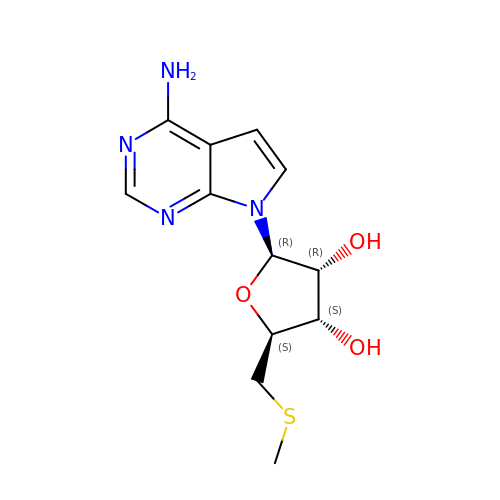2-(4-AMINO-PYRROLO[2,3-D]PYRIMIDIN-7-YL)-5-METHYLSULFANYLMETHYL-TETRAHYDRO-FURAN-3,4-DIOL | C12 H16 N4 O3 S | WBPLMFVTQMIPLW-MFYTUXHUSA-N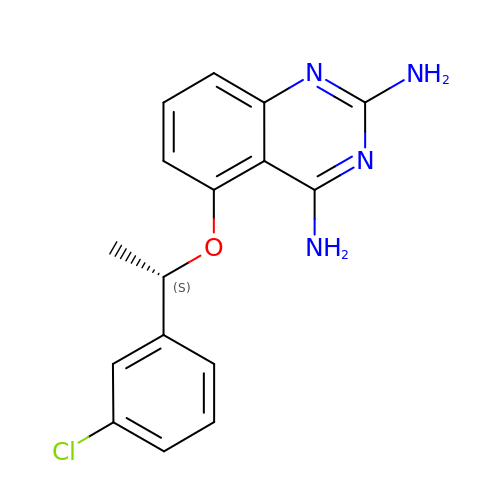5-[(1S)-1-(3-chlorophenyl)ethoxy]quinazoline-2,4-diamine | C16 H15 Cl N4 O | IDHINEMSCUFEIP-VIFPVBQESA-N> GPGMRVSGSASSQDIISRINSKNINNNDSNEVKRIKDALSIESKERILYPQNLSRDNLKQMARYVNNTYVHYSGNAVLLSACLHYNIHHRQDILSSKNTASPTVGLDSAIVDKIIFGHELNQSYSLNSIDEVEKEILNRYDIKRESSFIISAENYIAPIIGESGHDFNAVVISEY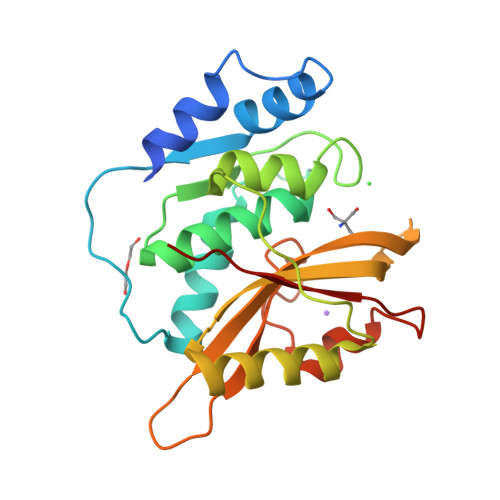DKKPYVQFIDSWKTSNILPSLQEIKKHFSSSGEFYVRAYDEKHD>[2x]GSHMASMTGGQQMGRGSAAQRQGALAIMSRVYVGSIYYELGEDTIRQAFAPFGPIKSIDMSWDSVTMKHKGFAFVEYEVPEAAQLALEQMNSVMLGGRNIKVGRPSNIGQAQPIIDQLAEEARAFNRIYVASVHQDLSDDDIKSVFEAFGKIKSATLARDPTTGKHKGYGFIEYEKAQSSQDAVSSMNLFDLGGQYLRVGKAVTPPMPLLTPATPG

Homologous to both U2AF65 and the yeast Mud2p, the Poly(U)-binding splicing factor 60 kDa (PUF60) shares domain features with U2AF65 by also containing two central RRMs and a C-terminal UHM. The most noticeable differences of domain structure between PUF60 and U2AF65 include the lack of the RS domain in PUF60 and a highly extended linker connecting the second RRM and UHM in PUF60. Although both U2AF65 and PUF60 are general splicing factors, the PUF60/U2AF65 ratio in cells influences alternative splicing patterns, suggesting PUF60 is implicated in alternative splicing. PUF60 appears to promote splicing at a weak 3’ splice site.

Herein is reported a 1.95 Å crystal structure of the two RRMs of PUF60 (PUF60 RRMs) in complex with a sequence from the adenovirus major late promoter (AdML) pre-mRNA 3’ splice site region (AdML3’). The structure reveals a homo-dimeric organization, where each participating PUF60 monomer captures a nucleic acid tract, and the PUF60 dimer places two nucleic acid tracts in antiparallel directionalities. Second, each monomer only binds to a short tract of nucleic acid using only the RRM1 but not the RRM2. Furthermore, the first position uracil bound to subunit A accepts a hydrogen bond from Lys-201 of subunit B, as discussed in the next section. RRM1 residues surrounding the uridine are shown in Fig 5, where Tyr-132 is the most outstanding feature that provides stacking for the uracil base. Therefore, UG is found bound to one subunit and UU bound to the other. Therefore, the bases of the wild-type sequence bound to the protein were assigned as U17-G18 on one side of the dimer, and UU from the polypyrimidine tract (PPT) on the other. Therefore, the looping in the wt dAdML3’ is deduced to occur between U17-G18 and the PPT. The Lys-201 side-chain from subunit B contacts U17 of dAdML3’, which is bound on the other side of the dimeric interface. This lysine donates a hydrogen bond to the 4-carbonyl oxygen of U17. The structure of dimeric PUF60 RRMs in complex with the AdML pre-mRNA 3’ ss region sequence suggests that PUF60 may also structure the pre-mRNA, albeit using a “looping” mechanism instead of “bending” as used by U2AF65.>MAESHWCYEVQAESSNYPCLVPVKWGGNCQKDRQSPINIVTTKAKVDKKLGRFFFSGYDKKQTWTVQNNGHSVMMLLENKASISGGGLPAPYQAKQLHLHWSDLPYKGSEHSLDGEHFAMEMHIVHEKEKGTSRNVKEAQDPEDEIAVLAFLVEAGTQVNEGFQPLVEALSNIPKP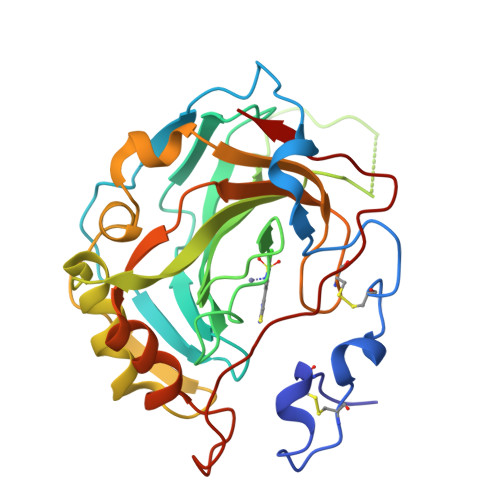EMSTTMAESSLLDLLPKEEKLRHYFRYLGSLTTPTCDEKVVWTVFREPIQLHREQILAFSQKLYYDKEQTVSMKDNVRPLQQLGQRTVIKS[4x]>[10x]MSPLRPQNYLFGCELKADKDYHFKVDNDENEHQLSLRTVSLGAGAKDELHIVEAEAMNYEGSPIKVTLATLKMSVQPTVSLGGFEITPPVVLRLKCGSGPVHISGQHLVAVEEDLEH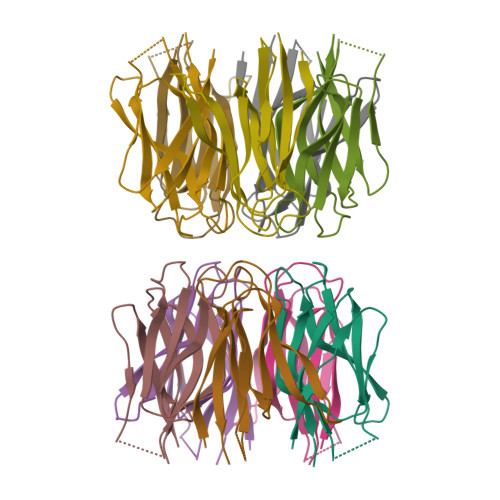HHHHH>MASKLRVVFATDEEIAAHEARLDLVQKKGGSCLWRATRESGSIGSMSEPRFVHLRVHSDYSMIDGPAKTAPLVKKAAALGMPALAITDFTNLCGLVKFYGAGHGAGIKPIVGADFNVQCDLLGDELTHLTVLAANNTGYQNLTLLISKAYQRGYGAAGPIIDRDWLIELNEGLILLSGGRMGDVGRSLLRGNSALVDECVAFYEEHFPDRYFLELIRTGRPDEESYLHAAVELAEARGLPVVATNDVRFIDSSDFDAHEIRVAI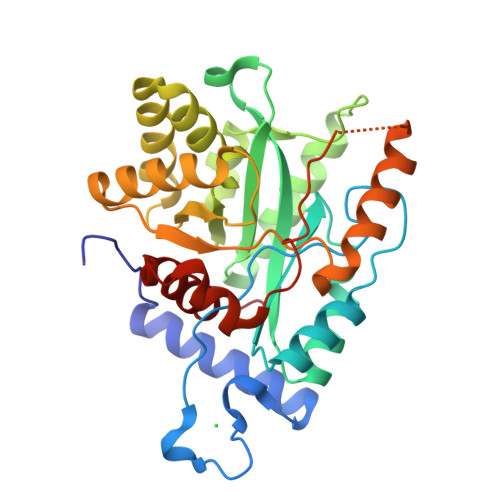HDGFTLDDPKRPRNYSPQQYMRSEEEMCELFADIPEALANTVEIAKRCNVT[4x]>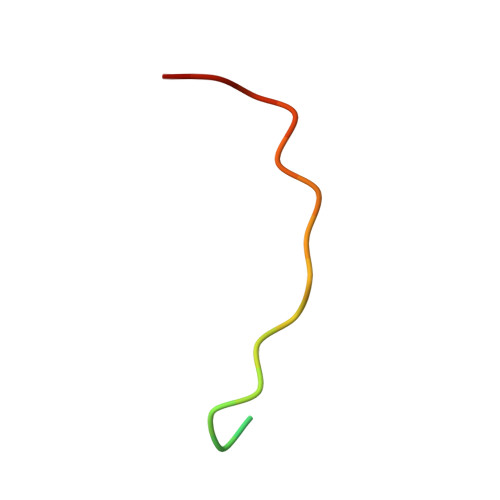 SKSRSTSSHGRRPLIRQDRIVG> RPIRLLPWLQVVKIGGRVM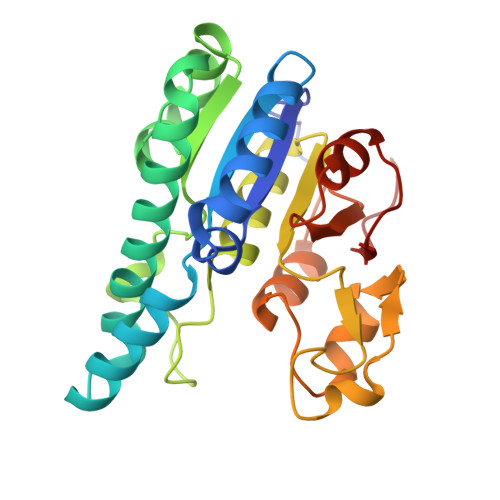DRGADAILPLVEELRKLLPEHRLLILTGAGVRARHVFSVGLDLGLPVGSLAPLAASEAGQNGHILAAMLASEGVSYVEHPTVADQLAIHLSATRAVVGSAFPPYHHHEFPGSRIPPHRADTGAFLLADAFGAAGLTIVENVDGIYTADPNGPDRGQARFLPETSATDLAKSEGPLPVDRALLDVMATARHIERVQVVNGLVPGRLTAALRGEHVGTLIRTGVRPA>MERINFIFGIHNHQPLGNFGWVFEEAYNRSYRPFMEILEEFPEMKVNVHFSGPLLEWIEENKPDYLDLLRSLIKRGQLEIVVAGFYEPVLAAIPKEDRLVQIEMLKDYARKLGYDAKGVWLTERVWQPELVKSLREAGIEYVVVDDYHFMSAGLSKEELFWPYYTEDGGEVITVFPIDEKLRYLIPFRPVKKTIEYLESLTSDDPSKVAVFHDDGEKFGVWPGTYEWVYEKGWLREFFDAITSNEKINLMTYSEYLSKFTPRGLVYLPIASYFEMSEWSLPAKQAKLFVEFVEQLKEEGKFEKYRVFVRGGIWKNFFFKYPESNFMHKRMLMVSKAVRDNPEARKYILKAQCNDAYWHGVFGGIYLPHLRRTVWENIIKAQRYLKPENKILDVDFDGRAEIMVENDGFIATIKPHYGGSIFELSSKRKAVNYNDVLPRRWEHYHEVPEATKPEKESEEGIASIHELGKQIPEEIRRELAYDWQLRAILQDHFIKPEETLDNYRLVKYHELGDFVNQPYEYEMIENGVKLWREGGVYAEEKIPARVE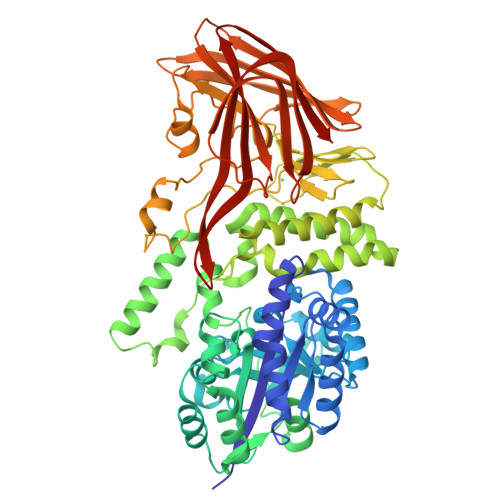KKIELTEDGFIAKYRVLLEKPYKALFGVEINLAVHSVMEKPEEFEAKEFEVNDPYGIGKVRIELDKAAKVWKFPIKTLSQSEAGWDFIQQGVSYTMLFPIEKELEFTVRFREL[2x]>[2x]GPRNLRVLLDTAIPPSFCDTVSSVLLDDFNMVSLIRTSPADSLATIKQDNAEIDIAITIDEELKISRFNQCVLGYTKAFVVAHPQHPLCNASLHSIASLANYRQISLGSRSGQHSNLLRPVSDKVLFVENFDDMLRLVEAGVGWGIAPHYFVEERLRNGTLAVLSELYEPGGIDTKVYCYYNTALESERSFLRFLESARQRLRELGRQRFDDAPAWQPSIVETAQRRSG

The eponymous PQS (Pseudomonas quinolone signal, 2‐heptyl‐3‐hydroxy‐4(1H)‐quinolone) and its biosynthetic precursor HHQ (2‐heptyl‐4‐quinolone) are both QS auto‐inducers acting as agonists on the transcriptional regulator PqsR (also referred to as MvfR). Among the various possible drug targets, PqsR is particularly attractive, as it is the essential transcriptional regulator of the PQS QS system serving major functions in PA virulence. Blocking this receptor results in affecting a number of down‐stream regulated processes such as virulence‐factor production, e.g., pyocyanin, biofilm formation or eDNA secretion. Due to its central role in virulence regulation, PqsR has been investigated in various studies as a promising new target for treating PA infections. It has been shown that small molecular agents, which act as inverse agonists on PqsR and thus inhibit QS, are able to reduce the production of the important virulence factor pyocyanin and the auto‐inducing alkylquinolones.

It became evident that the para‐substitution motif was suitable for growing. This was surprising, as this direction seemed to be occluded by residues Ile186 and Leu189 in the X‐ray structure and modeled binding mode. Nevertheless, we installed a number of substituents having various chemical properties in this 4‐position (shown in derivatives 9–15). Indeed, this attempt proved successful, as we discovered phenoxy‐modified compound 4, which showed a highly improved potency at IC50 of 11 × 10−9 m. The exploited growth vector was further endorsed by a co‐crystal structure of 4 in complex with the ligand binding domain of the transcriptional regulator PqsR91‐319. Herein, we observed the opening of an additional pocket upon binding. The para‐installed phenoxy moiety causes a 4 Å movement of Ile186 as measured by α‐carbon distance. Such observations of receptor flexibility and induced fit reshaping of the ligand‐binding site are fascinating and likely the reason for the observed non‐additive SAR. Optimized lead QSI 4 demonstrated high potency, suitable PK for pulmonary applications, a favorable safety pharmacology profile and was well tolerated in mice. In a murine lung‐infection model with a mucoid PA isolate, we successfully demonstrated the target engagement of the QSI 4 by recording a significant reduction of the proximal biomarkers HHQ, PQS, and HQNO.>APATETLDRRAALPNPYDDPFYTTPSNIGTFAKGQVIQSRKVPTDIGNANNAASFQLQYRTTNTQNEAVADVATVWIPAKPASPPKIFSYQVYEDATALDCAPSYSYLTGLDQPNKVTAVLDTPIIIGWALQQGYYVVSSDHEGFKAAFIAGYEEGMAILDGIRALKNYQNLPSDSKVALEGYSGGAHATVWATSLADSYAPELNIVGASHGGTPVSAKDTFTFLNGGPFAGFALAGVSGLSLAHPDMESFIEARLNAKGQQTLKQIRGRGFCLPQVVLTYPFLNVFSLVNDTNLLNEAPIAGILKQETVVQAEASYTVSVPKFPRFIWHAIPDEIVPYQPAATYVKEQCAKGANINFSPYPIA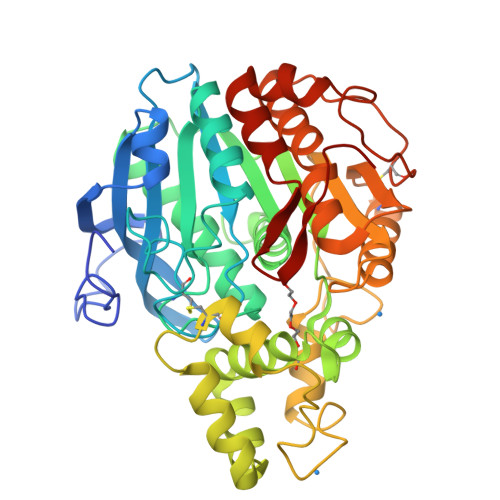EHLTAEIFGLVPSLWFIKQAFDGTTPKVICGTPIPAIAGITTPSADQVLGSDLANQLRSLNGKQSAFGKPFGPITPP[2x]> MGSRGSFVEMVDNLRGKSGQGYYVEMTVGSPPQTLNILVDTGSSNFAVGAAPHPFLHRYYQRQLSSTYRDLRKGVYVPYTQGKWEGELGTDLVSIPHGPNVTVRANIAAITESDKFFINGSNWEGILGLAYAEIARPDDSLEPFFDSLVKQTHVPNLFSLQLCGAGFPLNQSEVLASVGGSMIIGGIDHSLYTGSLWYTPIRREWYYEVIIVRVEINGQDLK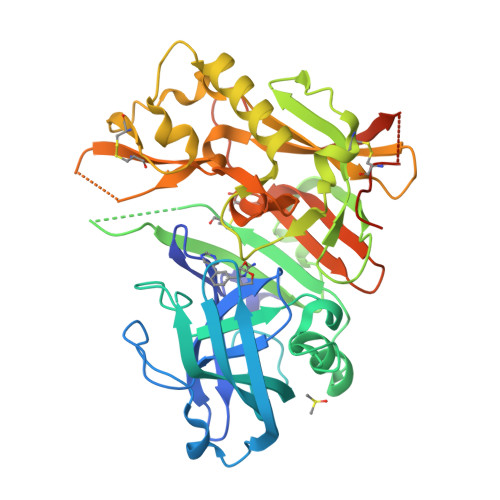MDCKEYNYDKSIVDSGTTNLRLPKKVFEAAVKSIKAASSTEKFPDGFWLGEQLVCWQAGTTPWNIFPVISLYLMGEVTNQSFRITILPQQYLRPVEDVATSQDDCYKFAISQSSTGTVMGAVIMEGFYVVFDRARKRIGFAVSACHVHDEFRTAAVEGPFVTLDMEDCGYNIPQTDESGNSHHHHHH> GPLGSKSSQVRTYPNGLIVEELSMGKPNGKRADPGKTVSVRYIGKLQKNGKIFDSNIGKSPFKFRLGIGSVIKGWDVGVNGMRVGDKRKLTIPPSMGYGVKGAGGQIPPNSWLT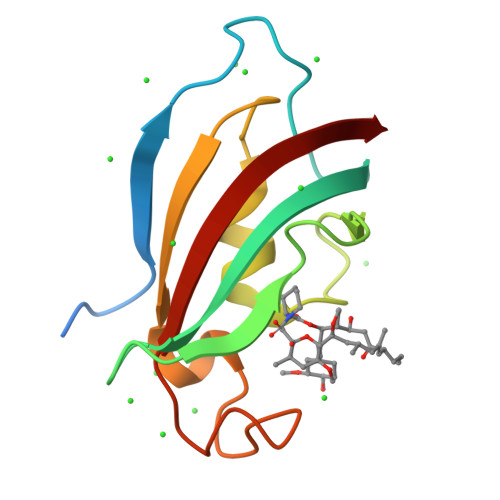FDVELINVQ2-{2-[4-(2-CARBAMIMIDOYLSULFANYL-ETHYL)-PHENYL]-ETHYL}-ISOTHIOUREA | C12 H18 N4 S2 | 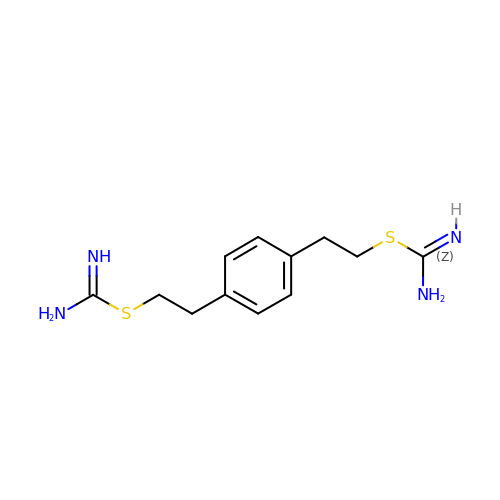FZWGDUUJDZCYJR-UHFFFAOYSA-N> GAHMNDIKQLLWNGELNVLVSIDPSFLMKGSPREIAVLRIRVPRETYLVNYMPLIWNKIKSFLSFDPLTDSEKYFWFEHNKTPIPWNYPVGVLFDCLAGKSATFTTSFENQVKDVLTFLRIHLVMGDSLPPTIIPIASSKTQAEKFWFHQWKQVCFILNGSSKAIMSLSVNEARKFWGSVITRNFQDFIEISNKISSSRPRHIPLIIQTSRTSGTFRISQPTISMTGVNPTLKDIEGDILDVKEGINGNDVMVICQGIEIPWHMLLYDLYSKLRSFDGFLYITLVPIKGGDKASSEL;> MGNFIITERKKAKEERSNPQTDSMDDLLIRRLTDRNDK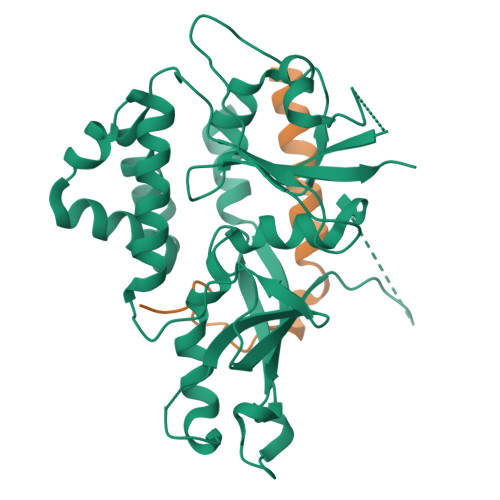EAHLNELFQDNSGAIGGNI> SNAMNIQILQEQANTLRFLSADMVQKANSGHPGAPLGLADILSVLSYHLKHNPKNPTWLNRDRLVFSGGHASALLYSFLHLSGYDLSLEDLKNFRQLHSKTPGHPEISTLGVEIATGPLGQGVANAVGFAMAAKKAQNLLGSDLIDHKIYCLCGDGDLQEGISYEACSLAGLHKLDNFILIYDSNNISIEGDVGLAFNENVKMRFEAQGFEVLSINGHDYEEINKALEQAKKSTKPCLIIAKTTIAKGAGELEGSHKSHGAPLGEEVIKKAKEQAGFDPNISFHIPQASKIRFESAVELGDLEEAKWKDKLEKSAKKELLERLLNPDFNKIA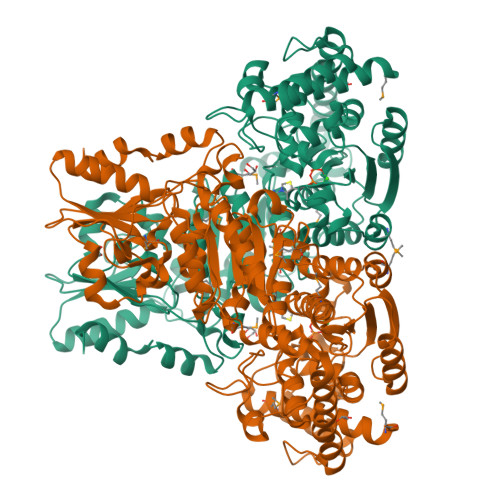YPDFKGKDLATRDSNGEILNVLAKNLEGFLGGSADLGPSNKTELHSMGDFVEGKNIHFGIREHAMAAINNAFARYGIFLPFSATFFIFSEYLKPAARIAALMKIKHFFIFTHDSIGVGEDGPTHQPIEQLSTFRAMPNFLTFRPADGVENVKAWQIALNADIPSAFVLSRQKLKALNEPVFGDVKNGAYLLKESKEAKFTLLASGSEVWLCLESANELEKQGFACNVVSMPCFELFEKQDKAYQERLLKGEVIGVEAAHSNELYKFCHKVYGIESFGESGKDKDVFERFGFSVSKLVNFILSK>MKKLLPILIGLSLTGFSAMSQAENLLQVYQQARISNPDLRKSAADRDAAFEKINEARSPLLPQLGLGADYTYTSGFRDYKDQNSNVTSGSLQLTQVLFDMSKWRALTLQEKAAGIQDVTYQTDQQTLILNTATAYFKVLAAIDTLSYTEAQKQAIYRQLDQTTQRFNVGLVAITDVQNARSQYDAVLANEVTARNDLDNAVEELRQVTGNYYPELASLNVDGFKTSKPQAVNALLKEAENRNLSLLQARLNQDLAREQIRQAQDGHLPTLDLNASSGVSNNRYSGSKSISQDADIGQNKIGLSFSLPLYQGGMVNSQVKQAQYNFVGASEQLESAHRSVVQTVRSSFNNVNASISSINAYKQAVVSAQSSLDAMEAGYSVGTRTIVDVLDATTTLYNAKQQLSNARYNYLINELNIKSALGTLNEQDLIALNNTLGKPISTSADSVAPENPQQDATADGYGNTTAAMKPASARTTTHSSGSNPFRQLEHHHHHH[3x];> MADNQPVPLTPAPPGMVSLGVNEN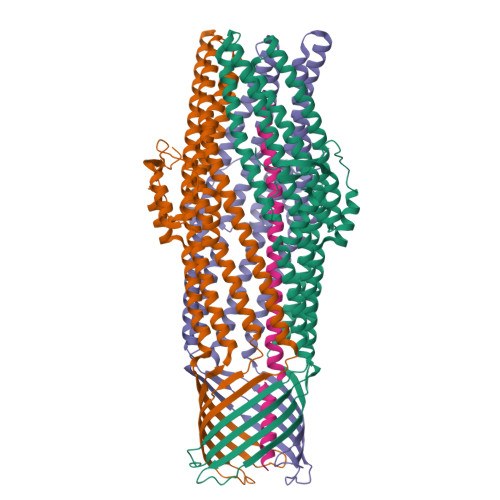GEEEMTVIGGDGSGTGFSGNEAPIIPGSGSLQADLGKKSLTRLQAESSAAIHATAKWTTENLAKTQAAQAERAKAAMLSQQAAKAKQAKLTQHLKDVVDRALQNNKTRPTVIDLAHQNNQQMAAMAEFIGRQKAIEEARKKAEREAKRAEEAYQAALRAQEEEQRKQAEIERKLQEARKQEAAAKAKAEADRIAAEKAEAEARAKAEAERRKAEEARKALFAKAGIKDTPGCLEHHHHHH>MASHMERDPQVAGLKVPPHSIEAEQSVLGGLMLDNERWDDVAERVVADDFYTRPHRHIFTEMARLQESGSPIDLITLAESLERQGQLDSVGGFAYLAELSKNTPSAANISAYADIVRER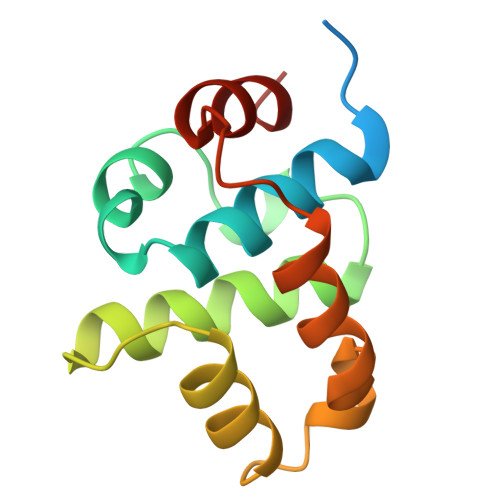[4x]> ASDYKDDDDKGALEVLFQGPSSPMAGNLVSWACKLCRSPEGFGPISFYGDFTQCFIDGVILNLSAIFMITFGIRDLVNLCKKKHSGIKYRRNWIIVSRMALVLLEIAFVSLASLNISKEEAENFTIVSQYASTMLSLFVALALHWIEYDRSVVANTVLLFYWLFETFGNFAKLINILIRHTYEGIWYSGQTGFILTLFQVITCASILLLEALPKKPLMPHQHIHQTLTRRKPNPYDSANIFSRITFSWMSGLMKTGYEKYLVEADLYKLPRNFSSEELSQKLEKNWENELKQKSNPSLSWAICRTFGSKMLLAAFFKAIHDVLAFTQPQLLRILIKFVTDYNSERQDDHSSLQGFENNHPQKLPIVRGFLIAFAMFLVGFTQTSVLHQYFLNVFNTGMYIKSALTALIYQKSLVLSNEASGLSSTGDIVNLMSVDVQKLQDLTQWLNLIWSGPFQIIICLYSLYKLLGNSMWVGVIILVIMMPLNSFLMRIQKKLQKSQMKYKDERTRVISEILNNIKSLKLYAWEKPYREKLEEVRNNKELKNLTKLGCYMAVTSFQFNIVPFLVSCCTFAVFVYTEDRALTTDLVFPALTLFNLLSFPLMIIPMVLNSFIEASVSIGRLFTFFTNEELQPDSVQRLPKVKNIGDVAINIGDDATFLWQRKPEYKVALKNINFQAKKGNLTCIVGKVGSGKTALLSCMLGDLFRVKGFATVHGSVAYVSQVPWIMNGTVKENILFGHRYDAEFYE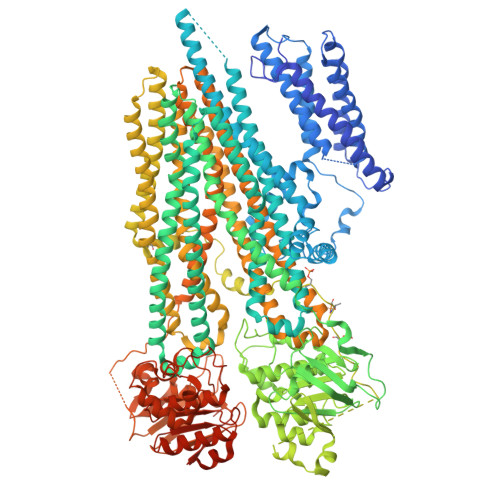KTIKACALTIDLAILMDGDKTLVGEKGISLSGGQKARLSLARAVYARADTYLLDDPLAAVDEHVARHLIEHVLGPNGLLHTKTKVLATNKVSALSIADSIALLDNGEITQQGTYDEITKDADSPLWKLLNNYGKKNNGKSNEFGDSSESSVRESSIPVEGELEQLQKLNDLDFGNSDAISLRRASDATLGSIDFGDDENIAKREHREQGKVKWNIYLEYAKACNPKSVCVFILFIVISMFLSVMGNVWLKHWSEVNSRYGSNPNAARYLAIYFALGIGSALATLIQTIVLWVFCTIHASKYLHNLMTNSVLRAPMTFFETTPIGRILNRFSNDIYKVDALLGRTFSQFFVNAVKVTFTITVICATTWQFIFIIIPLSVFYIYYQQYYLRTSRELRRLDSITRSPIYSHFQETLGGLATVRGYSQQKRFSHINQCRIDNNMSAFYPSINANRWLAYRLELIGSIIILGAATLSVFRLKQGTLTAGMVGLSLSYALQITQTLNWIVRMTVEVETNIVSVERIKEYADLKSEAPLIVEGHRPPKEWPSQGDIKFNNYSTRYRPELDLVLKHINIHIKPNEKVGIVGRTGAGKSSLTLALFRMIEASEGNIVIDNIAINEIGLYDLRHKLSIIPQDSQVFEGTVRENIDPINQYTDEAIWRALELSHLKEHVLSMSNDGLDAQLTEGGGNLSVGQRQLLCLARAMLVPSKILVLDQATAAVDVETDKVVQETIRTAFKDRTILTIAHRLNTIMDSDRIIVLDNGKVAEFDSPGQLLSDNKSLFYSLCMEAGLVNENGLVPRGSSAHHHHHHHHHHGA> MGYLHRVVEGLKANAGGEALVSADRRLTGAETLEEIHRTARALAAQGLRPGDGVVTLHGNGVEAVVLRIAVQLLGCRYAGLRPVFATREKANFLAEAEAAAFVYQPDMADEAAELLREVPTPRVLSLGPAPLGEDLVALAGAQSAEPVEFTADERAATAVGFTGGTTGRAKGVCRAPFDLEACLDASLTIFGEGPWRFLVCIPIADLGGEMAEWTLAAGGTVVLREDFEPADILATIGAERTTHVFCAPGWVYQLAEHPALADADLSSLTQIPYGGAPSTPARIADALEKLGRPLLVHCYGSQEGGWMTWLSAEDHVRADRYLLNSVGKALPGTEIAIRDQDGADLPVGTVGEVCVRSTMLMRGYWRLPELTAKTVRDGWLHTGDLGRLDTEGYLYLVDRAKDVIIVEAYNVYSQEVEHVLTGHPDVRYAAVVGVPDHDTTEAVYAAVVPAEGVGEIDVDELRALVRTTLGPVHEPKHLDVVDTIPTTPRGKPDK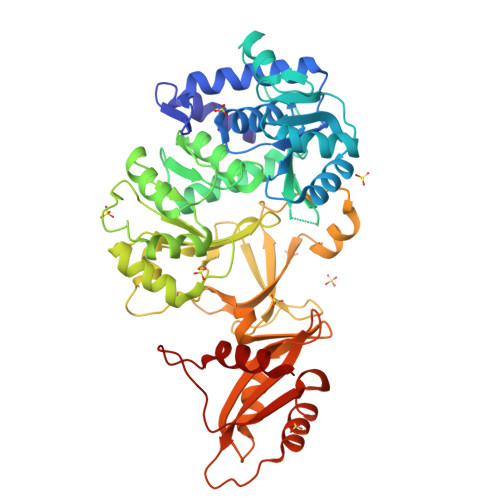SALRTRWRAAQRA>[8x]MHHHH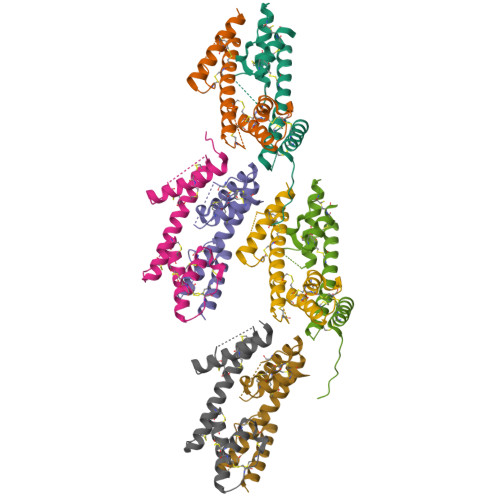HHMSTKDLIETCCAAGQQWAIDNDECQEIPENGAQSDICRIAQRQCCISYLKEKSCVAGVMGAKEGETCGAEDNDTCGVSLYKQCCDCCGLGLRVRAEGQSCESNPNLGYPCNHVMLSCCEG>GPGMDYQIDLVDPLTKVFADEVPDAWVVATQMVLQGEPLVLQLAYQRLRDDDASFSELTLATSLSAQCFEINQVPSQLPTWPHPDAR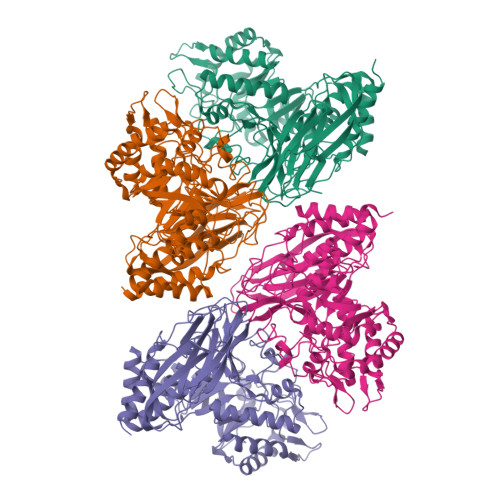YLRTTPGLFPDLLTPLTGPVRAYHGQVRALWLKIPTESLTPGSYELTITLTETASGQVVFSQTVPLTVAAAVAQPPRLHHTEWFSVDCLADYYHEAPYTPRLWAIIGNFMVFAHDEALMDTLLTPIFTPPLDTAVGATRTNVQLVQILPGTPYRFDWSRLRKWCQLAQQSGFAYLEMPPLFTQWGAQATPTITDTAGTALFGWHVPSTAPAYRAFLQALLPQLLAVLAEEGYDRDHLFFHLADEPNASTEDGYRAARAQVADLLDGLQVIDALSDVRFYENGLVPHPVVADDALAPFLAADAAPLWTYYCCAQTTAVPNRFFALRSYDNRVLGVLLYRHQIQGFLHWGFNFYNAQLSTRPIDPFAVTDAGGAFPSGDPFLVYPGADGQPLNSLRNEVQRLGFGDLAVLQQLEALKGRPFVERLIDVTAGMVPQFDDYPPDAGWLTRLHEKAVATLAAAAPAHKKE[4x]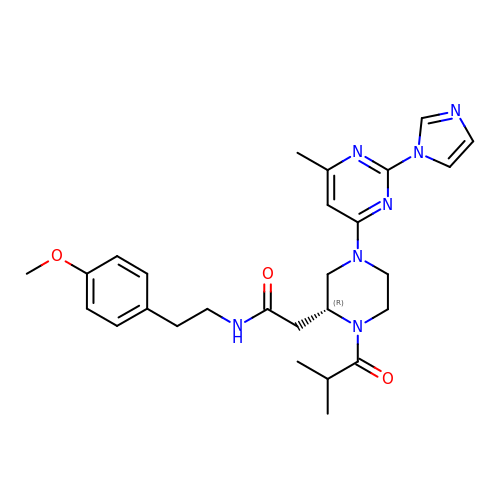2-{(2R)-4-[2-(1H-IMIDAZOL-1-YL)-6-METHYLPYRIMIDIN-4-YL]-1-ISOBUTYRYLPIPERAZIN-2-YL}-N-[2-(4-METHOXYPHENYL)ETHYL]ACETAMIDE | C27 H35 N7 O3 | TXTGZZWQXUQSGH-JOCHJYFZSA-N>[2x]MNTVRSEKDSMGAIDVPADKLWGAQTQRSLEHFRISTEKMPTSLIHALALTKRAAAKVNEDLGLLSEEKASAIRQAADEVLAGQHDDEFPLAIWQTGSGTQSNMNMN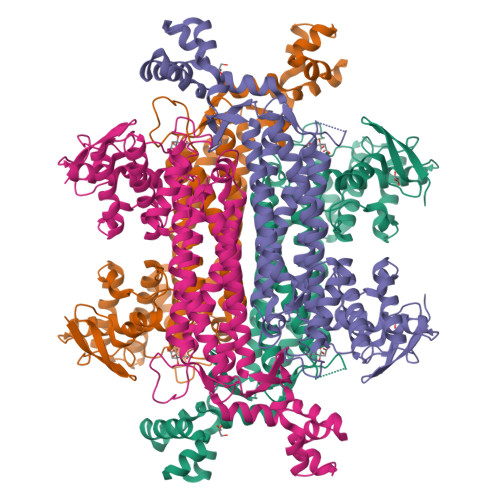EVLANRASELLGGVRGMEAKVHPNDDVNKSQSSNDVFPTAMHVAALLALRKQLIPQLKTLTQTLNEKSRAFADIVKIGRTHLQDATPLTLGQEISGWVAMLEHNLKHIEYSLPHVAELALGGTAVGTGLNTHPEYARRVADELAVITCAPFVTAPNKFEALATCDALVQAHGALKGLAASLMKIANDVRWLASGPRCGIGEISIPENEPGSSIMPGKVNPTQCEALTMLCCQVMGNDVAINMGGASGNFELNVFRPMVIHNFLQSVRLLADGMESFNKHCAVGIEPNRERINQLLNESLMLVTALNTHIGYDKAAEIAKKAHKEGLTLKAAALALGYLSEAEFDSWVRPEQMVGSMKAGRHHHHH>[4x]MNFGLFFLNFQLKGMTSEAVLDNMIDTIALVDKDEYHFKTAFVNEHHFSKNGIVGAPMTAASFLLGLTERLHIGSLNQVITTHHPVRIAEEASLLDQMSDGRFILGLSDCVSDFEMDFFKRQRDSQQQQFEACYEILNDGITTNYCYANNDFYNFPKISINPHCISKENLKQYILATSMGVVEWAAKKGLPLTYRWSDTLAEKE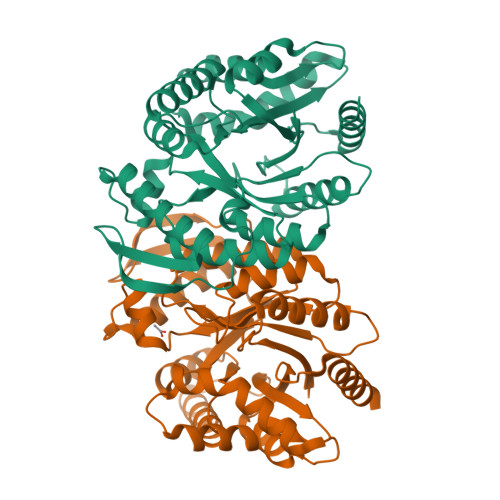NYYQRYLTVAAENNVDITHVDHQFPLLVNINPDRDIAKQEMRDYIRGYIAEAYPNTDQEEKIEELIKQHAVGTEDEYYESSKYALEKTGSKNVLLSFESMKNKAAVIDLINMVNEKIKKNL> MSFNESASIPTGLTYDDVLIIPQHSRVTSRKEVNTTTRLSRNVKLSIPIVASNMDTVCEQRMAVAMAREGGIGILHRFCSIEEQCAMLREVKRAQSFLIESPRIILPHETAREAWEGLNWKGRVGGVGCLLVVNCKNERKLLGIITRHDLKLADESTTVESLMTPVDKMVVSTNTSISLEEVTHLMRKGRTANVPIVGQNGQLLYLVTLSDVVKLRKN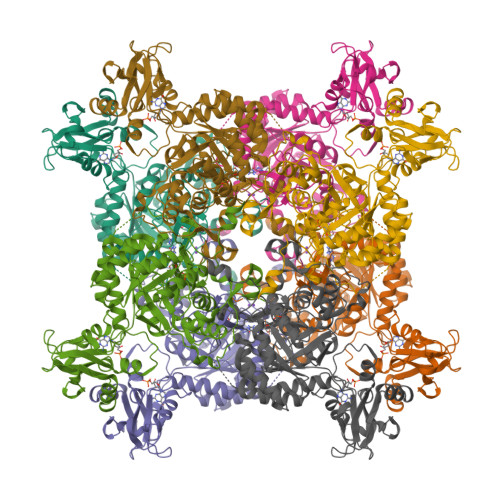KQASLDSRGRLLVGAAVGVKKDDMNRAIRLVEAGADVLVVDIAHGHSDLCINMVKRLKGDPRTASVDIIAGNIASAEAAEALIDAGADGLKIGVGPGSIAITRLVAGAGVPQLSAVLACTRVARRRGVPCIADGGLRTSGDISKAIGAGADTVMLGNMLAGTDEAPGRVLVKDGQKVKIIRGMAGFGANLSKAERERTQDEDVFSSLVPEGVEGSVACKGPVGPIVRQLVGGLRSGMSYSGAKSIEEMQRRTRFVRMTGAGLRESGSHGVAKLKLAAALEHHHHHH>[2x]MTTNVALVGLARDLAARAETGKPIRIGLIGAGEMGTDIVTQVARMQGIEVGALSARRLPNTFKAIRTAYGDEENAREATTESAMTRAIEAGKIAVTDDNDLILSNPLIDVIIDATGIPEVGAETGIAAIRNGKHLVMMNVEADVTIGPYLKAQADKQGVIYSLGAGDEPSSCMELI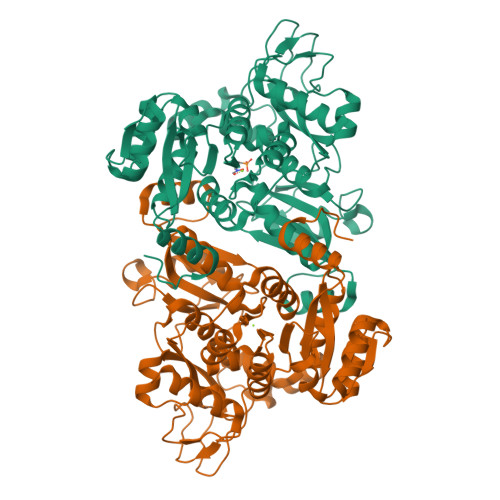EFVSALGYEVVSAGKGKNNPLNFDATPDDYRQEADRRNMNVRLLVEFIDGSKTMVEMAAIANATGLVPDIAGMHGPRASIDQLSHTLIPQAEGGVLSKSGVVDYSIGKGVSPGVFVVAKMDHPRLNERLEDLKIGKGPYFTFHRPYHLTSLEVPLTVARVVLHGKTDMVPLPKPVAEVCAVAKKDMQPGEHLDAIGQYCYRSWIMTVPEARAAKAIPCGLLQNGTVIAPIKKGELITYANAAPQPGSRIAELRALQDAMLGLEHHHHHH>[4x]MDKTTFRLLR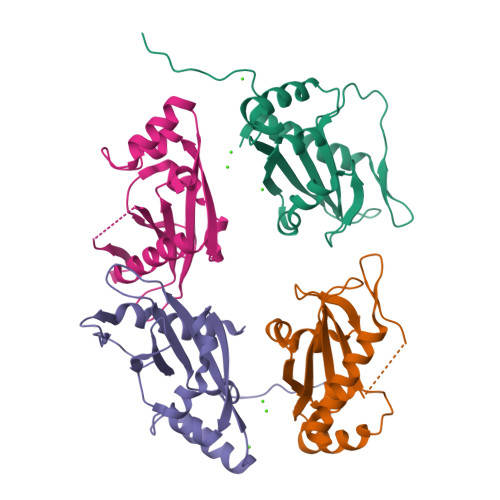GESNLFYTLAKWENNKISVELPENLDMQSPTMTLIYDETGKLLWTQRNIPWLIKSIQPEWLKTNGFHEIETNVDATSTLLSEDHSAQEKLKEVREDDDDAEMTHSVAVNIYPATARMPQLTIVVVDTIPIELKRSYMHHHHHH> MAQITLRGNAINTVGELPAVGSPAPAFTLTGGDLGVISSDQFRGKSVLLNIFPSVDTPVCATSVRTFDERAAASGATVLCVSKDLPFAQKRFCGAEGT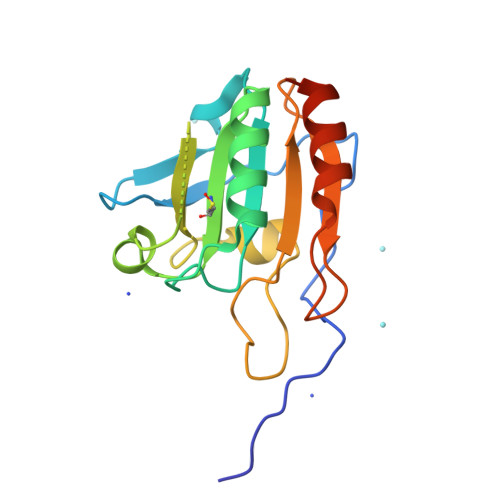ENVMPASAFRDSFGEDYGVTIADGPMAGLLARAIVVIGADGNVAYTELVPEIAQEPNYEAALAALGATSGSHHHHHH1H-imidazole-5-carbonitrile 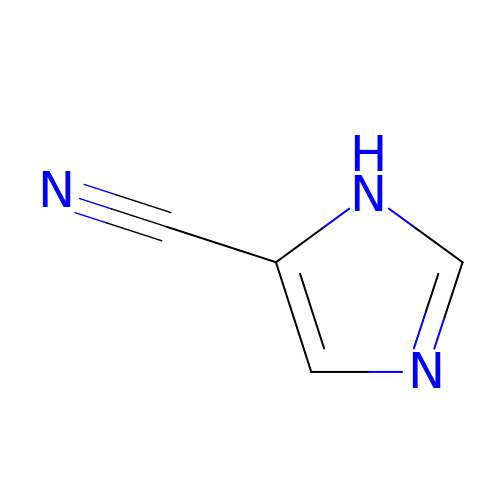| C4 H3 N3 | NWVGXXPWOYZODV-UHFFFAOYSA-N> KGRVCVTGGTGFLGSWIIKSLLENGYSVNTTIRADPERKRDVSFLTNLPGASEKLHFFNADLSNPDSFAAAIEGCVGIFHTASPIDFAVSEPEEIVTKRTVDGALGILKACVNSKTVKRFIYTSSGSAVSFNGKDKDVLDESDWSDVDLLRSVKPFGWNYAVSKTLAEKAVLEFGEQNGIDVVTLILPFIVGRFVCPKLPDSIEKALVLVLGKKEQIGVTRFHMVHVDDVARAHIYLLENSVPGGRYNCSPFIVPIEE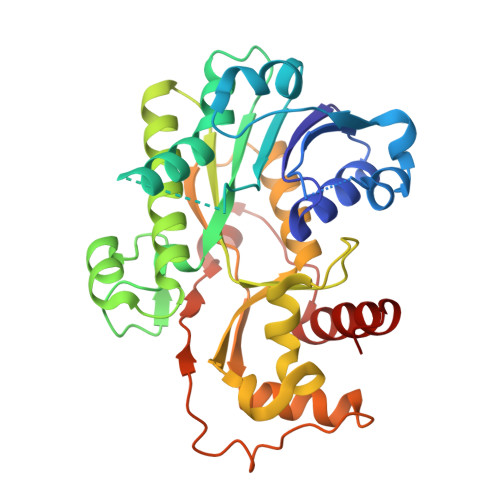MSQLLSAKYPEYQILTVDELKEIKGARLPDLNTKKLVDAGFDFKYTIEDMFDDAIQCCKEKGYL> IVGGQECKDGECPWQALLINEENEGFCGGTILSEFYILTAAHCLYQAKRFKVRVGDRNTEQEEGGEAVHEVEVVIKHN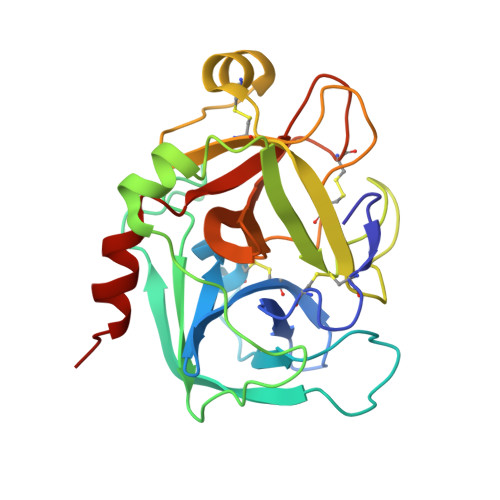RFTKETYDFDIAVLRLKTPITFRMNVAPACLPERDWAESTLMTQKTGIVSGFGRTHEKGRQSTRLKMLEVPYVDRNSCKLSSSFIITQNMFCAGYDTKQEDACQGDSGGPHVTRFKDTYFVTGIVSWGEGCARKGKYGIYTKVTAFLKWIDRSMKTR>[5x]MTVTYTARVAKARFGGFSKLLLLWRGSIYKLLWRELLCFLGLFMALSAAYRFVLTEEQKRYFEKLVLYCDRYASLIPVSFVLGFYVTLVVHRWWNQYLSMPLTDALMCVVVGTVHGHDERGRLYRRTLMRYAGLSGVLILRSVSTAVFKRFPTIDHVVEAGFMTREERKKFENLNSSYNKYWVPCVWFCNLAAQARREGRIRDNGAFKLLLEELNVFRSKCGMLFHYDWISVP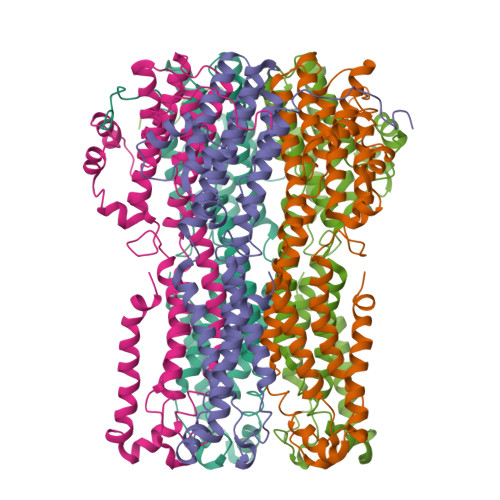LVYTQVVTIAVYSYFLACLIGRQFLDPAQGYKDHDLDLCVPIFTLLQFFFYAGWLKVAEQLINPFGEDDDDFETNFLIDRCFQVSMLAVDEMYDDLAMLEKDLYWDAAEARAPYTAATAFLMQQPSFQGSTFDITLAKEDMQFQRQDGLEAPLNEAHGDFLQRLLPVGTGMGTGGLL> GAFARDPTQFEERHLKFLQQLGKGNFGSVEMCRYDPLQDNTGEVVAVKKLQHSTEEHLRDFEREIEILKSLQHDNIVKYKGVCYSAGRRNLKLIMEYLPYGSLRDYLQKHKERI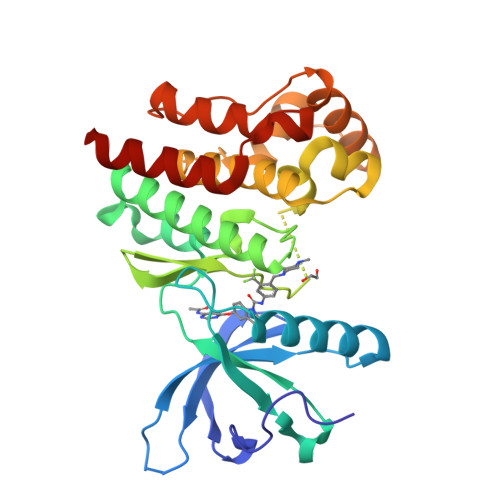DHIKLLQYTSQICKGMEYLGTKRYIHRDLATRNILVENENRVKIGDFGLTKVLPQDKEYYKVKEPGESPIFWYAPESLTESKFSVASDVWSFGVVLYELFTYIEKSKSPPAEFMRMIGNDKQGQMIVFHLIELLKNNGRLPRPDGCPDEIYMIMTECWNNNVNQRPSFRDLALRVDQIRDNMAG(1R,3S)-3-[(E)-({3-hydroxy-2-methyl-5-[(phosphonooxy)methyl]pyridin-4-yl}methylidene)amino]-4-oxocyclopentane-1-carboxylic acid | C14 H17 N2 O8 P | 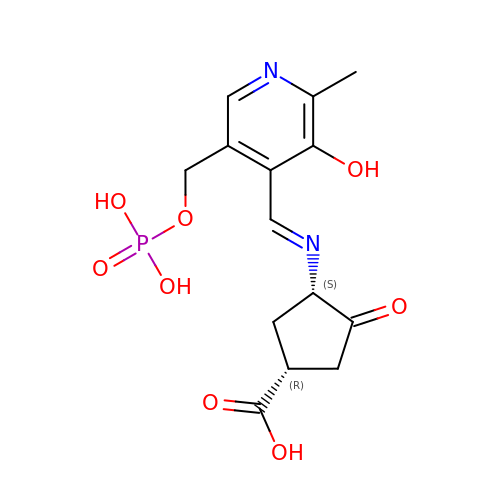XLGFWCHBZWEILL-SNTOBFBISA-N Unlike Halobacteriovorax species that are intracellular predators, strain CF6-2 is an extracellular predator, which kills Gram-positive bacteria by secreting an extracellular protease, pseudoalterin, that degrades the PG in the prey’s cell wall. (ii) Pseudoalterin can bind to the glycan strand of Gram-positive bacterial PG with its C-terminal domain and degrade the PG peptide with its catalytic domain. Pseudoalterin preferred to cleave the bonds with Gly/Ala at P1 and P1′ positions and, to a lesser extent, to the bonds with larger amino acids at these positions. In the meantime, the released glycine and glycine-enriching oligopeptides from the degradation of Gram-positive bacterial PG induce the synthesis of pseudoalterin in strain CF6-2, and then the synthesized pseudoalterin is secreted through the T2SS of strain CF6-2.

To better understand the molecular interaction between pseudoalterin and PG, the crystal structure of pseudoalterin was determined to 1.9 Å. The sequence identity of pseudoalterin to the M23 peptidases LasA and lysostaphin is 54% and 15%, respectively. The catalytic domain of pseudoalterin, comprising five β-strands and four connecting loops (loop 1–loop 4), is quite similar to those of LasA and lysostaphin, with a root mean square deviation (RMSD) of 0.64 and 4.0 Å, respectively. H21, D34, and H120 chelating the zinc ion in pseudoalterin are equivalent to H210, D214, and H293 that chelate the zinc ion in LytM21. Among them, either H79 or H118 can act as a general base/acid in PG hydrolysis based on sequence alignment of pseudoalterin with its homologs (LasA, LytM, lysostaphin, and ALE-1), and mutation of these two residues to alanine almost completely abolished pseudoalterin activity to PG. In the model of the pseudoalterin: (NAG–NAM)2 binary complex (NAG, N-acetylglucosamine; NAM, N-acetylmuramic acid), the glycan strand (NAG–NAM)2 interacts with the C-terminal domain. Analysis of the model indicated that (NAG–NAM)2 interacts with the C-terminal domain mainly by forming H-bonds with the residues H133, N134, Y136, R141, D143, N154, Y157, E159, R163, and R164. The catalytic cavity of pseudoalterin is similar to those of LasA and LytM, and more open than that of lysostaphin, which suggests that, like these homologs, pseudoalterin also prefers to bind Gly/Ala. In addition, compared to LasA, the side chain of Q113 of loop 3 of pseudoalterin makes the S1 pocket much deeper, and may be capable of orienting the long side chain of amino acids. Thus, in addition to Gly and Ala, the deeper and more open catalytic cavity of pseudoalterin may accommodate residues with a longer side chain such as Lys and Glu in PG.

> ATFTMNLPWSQGYYWYSGGAHSNTGSGYPYSSLDFNNGSGGWGSNTPWVQAAHGGVITRFSSCNIRVTHSSGFATNYYHMSNLQYNNGDTVQPGTLLGRYANSYNQALCEGGQSSGPHVHFTLLQNGQQVSLHNRYISNYRIDVGNSNYDSNCNNFYFERNGRRTCAWRPLYR propane-1,1-diol | C3 H8 O2 | 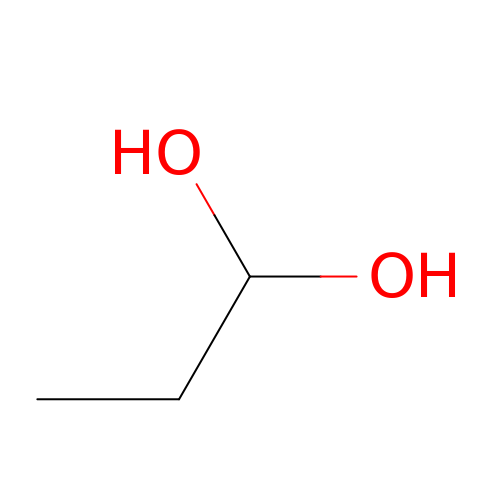ULWHHBHJGPPBCO-UHFFFAOYSA-N>AEGDDPAKAAFNSLQASATEYIGYAWAMVVVIVGATIGIKLFKKFTSKAS[25x];>[5x]MEQVADFDTIYQAMIQISVVLCFALGIIAGGQR;>MSVLVYSFASFVLGWCLRSGITYFTRLMETSS[5x]

Filamentous bacteriophages package their circular, single stranded DNA genome with the major coat protein pVIII and the minor coat proteins pIII, pVII, pVI, and pIX. Here, we report the cryo-EM structure of a ~500 Å long bacteriophage M13 mini variant. The distal ends of the mini phage are sealed by two cap-like complexes composed of the minor coat proteins. We further performed local refinements of the mini phage by dividing the particle into the top, middle and bottom three segments.

The top spheric cap is a complex of pIX, pVII, and pVIII. The five pVII molecules form a symmetric plug-like pentamer that are located at the top middle of the cap. The five pVIIs mainly interact with each other through hydrophobic residues, including F7, I10, A13, M14, L21, A24, L25, and A29. The 5 pIX molecules of the protein layer 2 assemble around the pVII pentamer. Interactions between pIX and pVII mainly involve hydrophobic interactions, hydrogen bonds, and salt bridges. The molecules from the first layer of pVIII (layer 3) are inserted in between the pIX molecules and have a completely different contact environment compared to the pVIII molecules from other layers. The bent angle (~34° from the main axis of the virion) of the pVIII in layer 3 is significantly larger than those (~21°) of the pVIIIs in layers 4–5 and the middle part of the particle, due to the specific environment of pVIII molecules in the layer for establishing interactions with pIX and pVII. The cap constituted by pVII, pIX, and pVIII has a unique lumen that is decorated with four positively charged residues, including R33 of pVII, K40, K43, K48 of pVIII and one negatively charged residue, E29 of pIX. Among these, residues R33 of pVII and E29 of pIX are in proximity to the encapsidated DNA genome, indicating that these residues could be involved in direct interactions and specific recognition of the genome packaging signal, which was supposed to have a hairpin structure. Further mutagenesis studies of residues E29 of pIX and R33 of pVII showed that these residues are essential for the assembly of living viruses.> RPK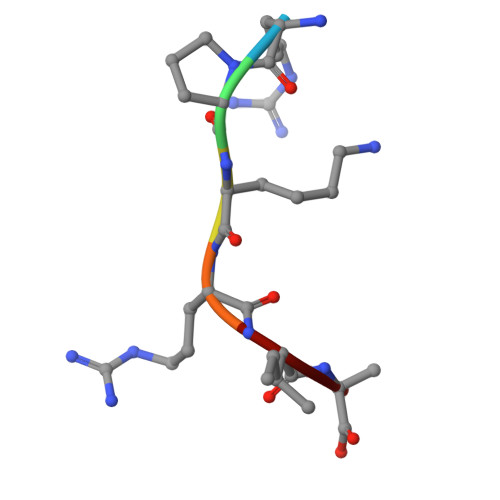RIA>[2x]GKE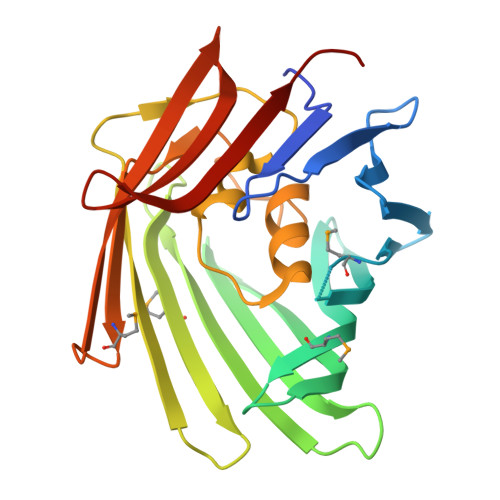KKADTYVTKVTDLTGEEEQVLKLEYDRDGKIIKYGDTPVRYEGDQITIGQMNCLNTGNKLCNVTFQIGKGKARESRARCMLKVGEEVYEADKQTVYDYKGDTIFINSDYRATSDYRFLKKVQGKYVFDQLGRLKEVMTVFTEANDSVSSCHTYYNYDNNINYQANLNLQAYVIDYDGVDSFFYFLLNLGQLRNRTALPNDIGYCMNHGLSTYNVHANYRLDDENPVRIEVLYNYTKLLSRIDLSYNPLN N-(6-{2-[2-(2-amino-3-{3-[(3,3-dimethylbutyl)amino]-3-oxopropyl}quinolin-6-yl)phenyl]ethyl}pyridin-3-yl)-4-fluorobenzamide 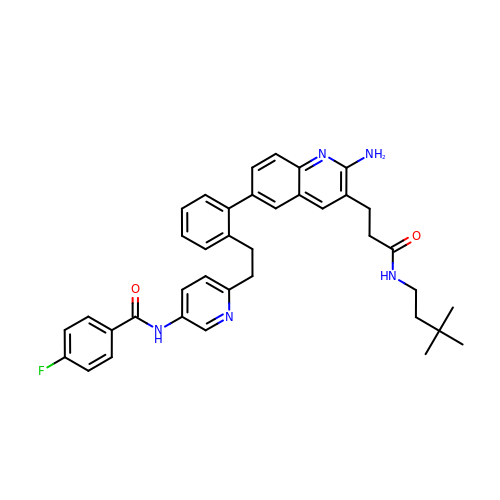| C38 H40 F N5 O2 | RTOUKFMBOVMEOT-UHFFFAOYSA-N> MTAVRRSTRIRTKSQVIEEDYDDEQNTSAQHVESDKITAKTQHEEEEEQDTGESEESSSEDDYEDQDDDDYVDTATAKRKSRKRKPKSASNTSSKRQKKKPTSAQKSAVSHAPAYHRSKKDQDQYLEIAKDFQPTELFDILSTSEDVSIEELLREWLETYSENRDKFLQEFINLLLNCCGSVARVEDHDVHSNESSNETIGEIQLLFQRQKLHEFYLLISKENKKRKNFKMGPLYQNFAEFMTKLLEVANDLQLLYVESDEDDTQIVTGNLVLDLLTWLSSFSVCKIRCFRYISTLTLYLFQDYLTQQAVNLEKNYLAKLSKQLSLEEKKKRPNNKTLEKLESTIAETQGSKVVIDSIIDNIV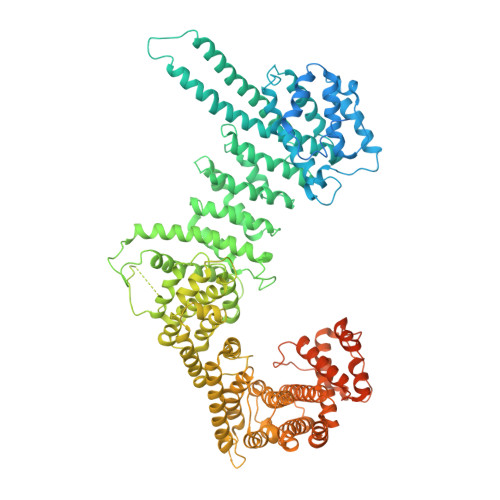KLCFVHRYKDVSDLIRSESMLHLSIWIKNYPEYFLKVTFLKYFGWLLSDNSVSVRLQVTKILPHLIIQNHNSKSTDNSAIRQVFERFKTKILEVAIRDVNLDVRIHSIQVLTEASSLGYLDDSEILIISSLMFDEEFDPFKTSSFNKRSKFLSTVAKFLARVIKEKFDEFIKTHEDLPKEVDGLEVGPVVQVGIFIKILNDSLIYHLKDCAEVDSRTKIRMLTQAAEFLSPYISTHLKTICNLLISDTESNELIQKLQNSANNNSDDEDVDDEELDITPLFPIDRNSTILYLNVFHGLCAGANNPKIQTKDSVKEIVLPLFYDLLNAASIESADILCPLLESFITFSLDDWISIGYETELKKITDKTIKAFMDSTIGNSKVDMKYDIFAKFIHHIHHFEKKELQEKFLNQIATLKIHLKKFLQEKMDPNNSRDDYKDLTCSLYELYINKLTILGRDYPIEVDEELLQLFLNNFVSRIPIMFQDFDDSTAQEINFKMLVLLATWNLEKWREIIEKVRDYENSISKDLRSVWKPIAAIIGRLNTLVISLAATNETFENINSLFYLKWSACTSLMDIIVAIKIFELKLPADATTWRYSMSEQFPFYLHDNASKVLLKIFLYLESLFAKQVDVQLERVADEDANLNDLPETGFFENIETEFLLFTVKLKGLMKLNILDERFASRVALNKEKLGPLFKKIVDDTIMENPEPNKKNIQKAKSNQTQREKAPLQPNSERETDHANTENNDPDIPMTIDLEPIEESSQNNSELAPIEEHPTVVDAIDNSDEITQD> MALSDADVQKQIKHMMAFIEQE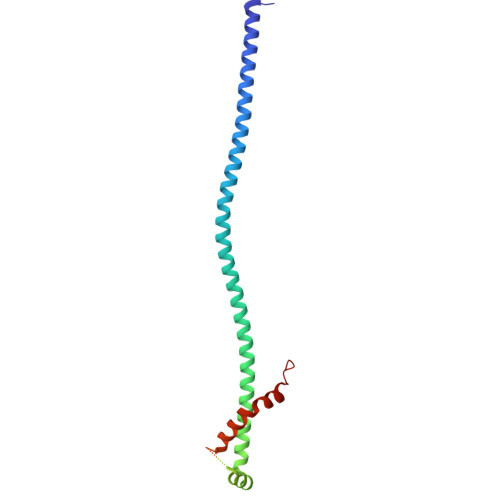ANEKAEEIDAKAEEEFNIEKGRLVQTQRLKIMEYYEKKEKQIEQQKKIQMSNLMNQARLKVLRARDDLITDLLNEAKQRLSKVVKDTTRYQVLLDGLVLQGLYQLLEPRMIVRCRKQDFPLVKAAVQKAIPMYKIATKKDVDVQIDLEAYLPEDIAGGVEIYNGDRKIKVSNTLESRLDLIAQQMMPEVRGALFGANANRKFLD>[2x]NRGVLKVYLDYRRKNFNFLHNSTKMFLDNLERVLIVTGFPIPPMMVAETDGPPGALAI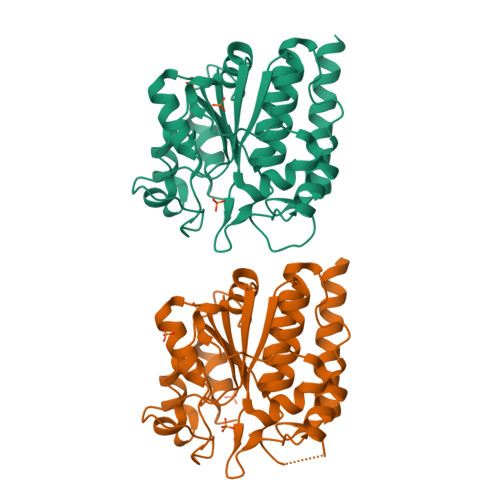YRAVEMLGGKAEILTYSEVEKALEPFGVSLARTPEPEDYSLIISVETPGRAADGRYYSMSALEIKRDPLDGIFLKARALGIPTIGVGDGGNEIGMGKIRELVVGHVPHGEKIASVVETDELIVSAVSNWGAYGLVAQASIEVGRNLLEGWDERRVIEAISSAGLIDGVSKTLAPSVDGIRLMVHEGIVELLKAVVDEAIKL> LSNGLGRTPQMGWSSWNHFACNIEEKEIRETADAMVSTGLASLGYEYINIDDCWAELNRDSQGNMVPKGSTFPSGIKALADYVHSKGLKLGIYSDAGSQTCSKQMTGSLGHEEQDAKTFASWGVDYLKYDNCNNENRSPRERYPIMAKALKNSGRAIFYSLCEWGDDDPATWASSVGNSWRTTGDISDNWDSMTSRADMNDEWASYAGPGGWNDPDMLEVGNGGMTTAEYRSHFSIWALAKAPLIIGCDLRSMDQTAHEILSNKEVIAVNQDKLGVQGKKVKQNGDLEVWAGPLSGKRVALVLWNRSSSKADITAYWSDIGLDSS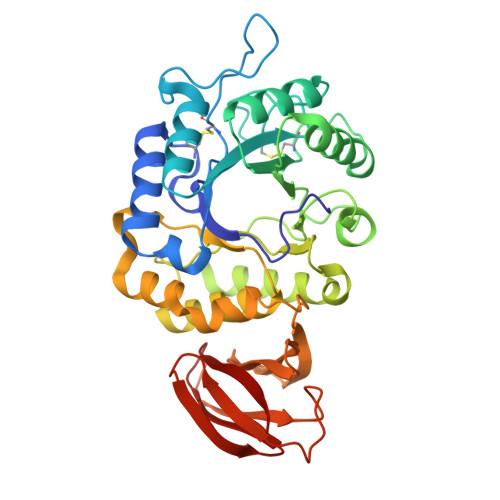TVVDARDLWAHSTKGSVKGQISASIDSHDCRMYVLTPK>ANIVGGIEYS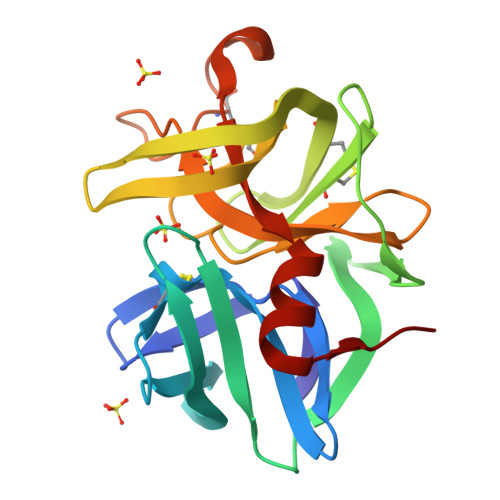INNASLCSVGFSVTRGATKGFVTAGHCGTVNATARIGGAVVGTFAARVFPGNDRAWVSLTSAQTLLPRVANGSSFVTVRGSTEAAVGAAVCRSGRTTGYQCGTITAKNVTANYAEGAVRGLIQGNACMGRGDSGGSLITSAGQAIGVMSGGNVQSNGNNCGIPASQRSSLFERLQPILSQYGLSLVTG[2x]A key part of this process would have been the nonenzymatic template directed polymerization of activated RNA nucleotides. We therefore chose to use the oligoribonucleotide 5′-CCCGACUUAAGUCG-3′ which contains four locked nucleic acid (LNA) residues, denoted by italics. By obtaining crystal structures at various times after the initiation of the reaction, we were able to capture a sequence of molecular ‘snapshots’ that follow the progress of the nonenzymatic RNA polymerization reaction.

Having obtained crystals of the RNA-dGMP complex, we sought to replace the bound dGMP residues with purified imidazolium-bridged diguanosine intermediate (Gp-AI-pG). No Mg2+ was included in either the crystallization or soak buffers, to improve the solubility and stability of the Gp-AI-pG. The Gp-AI-pG molecule was observed by crystal structure determination to bind the template in place of dGMP, and optimal structures were obtained after 4 hr of soaking the crystals in the exchange buffer. In the crystal structures, Gp-AI-pG binds the -CC template at both ends of the RNA duplex exclusively through Watson-Crick base-pairing, with hydrogen bond distances of 2.8 to 3.3 Å. Similar to our previous analysis of the analog GpppG, the Gp-AI-pG intermediate is well-ordered and displays only the C3′-endo sugar conformation. The 4.6 Å distance between the 3′-hydroxyl and the phosphate of the nucleotide in the +1 position is shorter than the corresponding 6 to 6.5 Å distance for the 2′-hydroxyl, consistent with the observed 3′ regioselectivity of polymerization using 2-methyl and 2-aminoimidazole activated monomers. The electron density corresponding to the phosphate-aminoimidazole-phosphate bridge suggests that its structure is stabilized by hydrogen bonds between the 2-amino group of the imidazolium moiety and the non-bridging oxygen atoms of the flanking phosphates. For the 3′-hydroxyl, the distance to the phosphorous atom is 4.6 Å in both orientations, but the angle of attack changes from 170° when the 2-amino points toward the minor groove, to 132° when it points towards the major groove. A key difference is the decreased distance between the 3′-hydroxyl of the primer and the phosphate in the +1 position, from 6.5 Å for bound dGMP to 4.6 Å for template-bound Gp-AI-pG. In contrast, when Gp-AI-pG was soaked into the crystal without Mg2+, no reaction was observed.

>NNNGACUUAAGUCG[2x]>[2x]MISNSSAESISAPPNDSTIPHLAIDPFSLDFFDDPYPDQQTLRDAGPVVYLDKWNVYGVARYAEVHAVLNDPTTFCSSRGVGLSDFKKEKPWRPPSLILEADPPAHTRPRAVLSKVLSPATMKTIRDGFAAAADAKVDELLQRGCIDAIADLAEAYPLSVFPDAMGLKQEGREHLLPYAGLVFNAFGPPNELRQTAIERSAPHQAYVNEQCQRPNLAPGGFGACIHAFTDTGEITPDEAPLL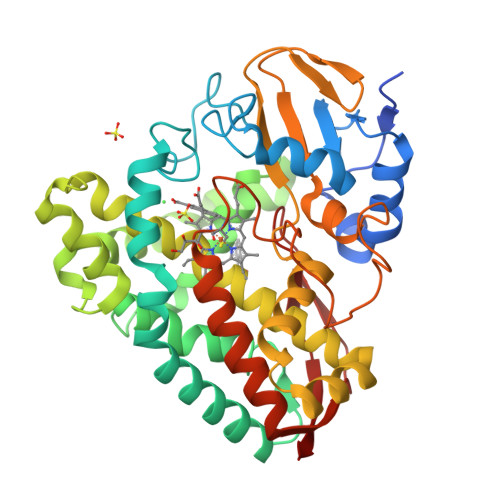VRSLLSAGLDTTVNGIGAAVYCLARFPGELQRLRSDPTLARNAFEEAVRFESPVQTFFRTTTREVELGGAVIGEGEKVLMFLGSANRDPRRWSDPDLYDITRKTSGHVGFGSGVHMCVGQLVARLEGEVMLSALARKVAAIDIDGPVKRRFNNTLRGLESLPVKLTPA Kaposi's sarcoma‐associated herpesvirus (KSHV), a member of the human γ‐herpesviruses family, exhibits extensive cellular tropism and is associated with Kaposi's sarcoma and various B‐cell malignancies. Similar to other herpesviruses, KSHV depends on the envelope glycoprotein B (gB) for host receptor recognition and membrane fusion initiation, making gB a prime target for antiviral antibody or vaccine development. As the fusion protein, gB mediates viral membrane fusion with the host membrane, triggered by signal from the gH/gL heterodimer—a mechanism consistent across herpesviruses. In this study, the high‐resolution cryo‐electron microscopy (cryo‐EM) structure of KSHV gB is presented, revealing a unique trimeric conformation resembling the postfusion state observed in other herpesviruses.

We determined the cryo‐EM structure of the KSHV gB ectodomain at a resolution of 3.26 Å. This breakthrough was made possible by a novel construct, gB653‐mut, which incorporates strategic substitutions from the FL from HSV‐1 gB and mutations in the furin site. The KSHV gB653‐mut ectodomain, analyzed in our study, adopts the well‐characterized postfusion gB structure, forming a homo‐trimeric, rod‐like spike. This structure measures ≈170 Å in height, with a major and minor radius of ≈35 Å and 24 Å, respectively. The structure consists of five distinct domains (Domain I through V or DI‐DV), spanning residues 53–653. However, a certain region (411–453) was unresolved in the cryo‐EM map. We identified three pairs of intramolecular disulfide bonds (C68‐C528 in DIV, C85‐C484 in DIII, and C315‐C362 in DII) and observed no inter‐chain disulfide bonding, indicating a tight but flexible trimeric assembly. The FLs of the wild‐type KSHV gB consist of two loops, LT‐FL1 and WFPGI‐FL2, characterized by high hydrophobicity (L‐FL1; W, F, P, G, I‐FL2), whereas the KSHV gB653‐mut FL, HR‐FL1 and RVEA‐FL2 from HSV‐1 gB, incorporate with polar amino acid (H, R‐FL1; R, E, T‐FL2). In detail, the presence of acidic (E211‐FL2) and basic amino acids (R129‐FL1; R209‐FL2) renders the lowest bottom of KSHV gB653‐mut highly hydrophilic, with a negatively charged bottom tip due to the carboxyl group of glutamic acid, surrounded by positively charged side chains from the amidogen of arginine. This may stabilize the gB653‐mut ectodomain in a solvent environment during purification, compared to the wild‐type construct. Domain III (DIII) also consists of two parts, DIIIa (I72‐ Y92) and DIIIb (D454‐C528), featuring a central, long helix forming a trimeric, left‐handed bundle, providing strong interchain contacts.

>MTPRSRLATLGTVILLVCFCAGAAHSRGDTFQTSSSPTPPGSSSKAPTKPGEEASGPKSVDFYQFRVCSASITGELFRFNLEQTCPDTKDKYHQEGILLVYKKNIVPHIFKVRRYRKIATSVTVYRGHRESAITNKYELPRPVPLYEISHMDSTYQCFSSMKVNVNGVENTFTDRDDVNTTVFLQPVEGLTDNIQRYFSQPVIYAEPGRVEATYRVRTTVNCEIVDMIARSAEPYNYFVTSLGDTVEVSPFCYNESSCSTTPSNKNGLSVQVVLNHTVVTYSDRGTSPTPQNRIFVETGAYTLSWASESKTTAVCPLALWKTFPRSIQTTHEDSFHFVANEITATFTAPLTPVANFTDTYSCLTSDINTTLNASKAKLASTHVPNGTVQYFHTTGGLYLVWQPMSAINLTHAQGDSGNPTSSPPPSASPMTTSASRGGSGGASTAAAGGGGSTDNLSYTQLQFAYDKLRDGINQVLEELSRAWCREQVRDNLMWYELSKINPTSVMTAIYGRPVSAKFVGDAISVTECINVDQSSVNIHKSLRTNSKDVCYARPLVTFKFLNSSNLFTGQLGARNEIILTNNQVETCKDTCEHYFITRNETLVYKDYAYLRTINTTDISTLNTFIALNLSFIQNIDFKAIELYSSAEKRLASSGSHHHHHH[3x]5-amino-2,4,6-tribromobenzene-1,3-diyl dihydroperoxide | 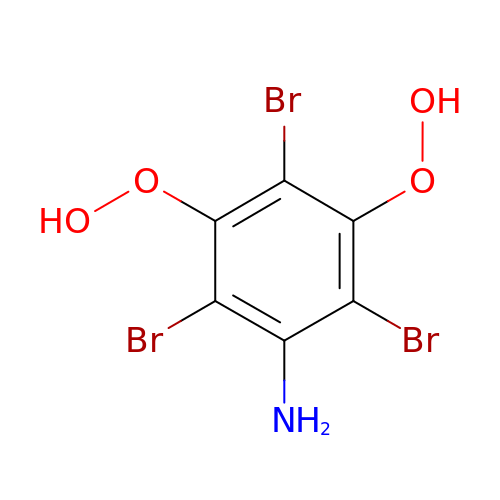C6 H4 Br3 N O4 | LZZXDGTUENOCKF-UHFFFAOYSA-N>ATYAAASSALVPRGSHMYAPKLQGPVAVYTWEGNQVNITCEVFAYPSATISWFRDGQLLPSSNYSNIKI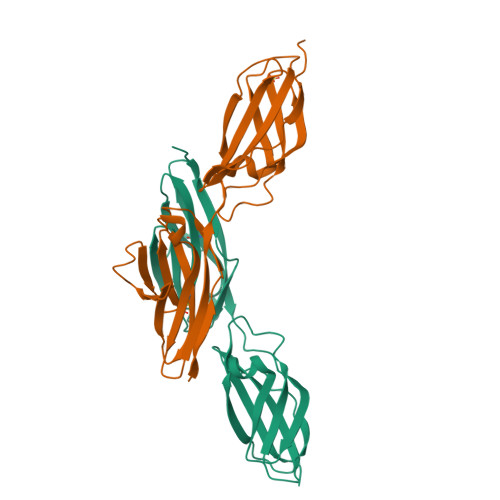YNTPSASYLEVTPDSENDFGNYNCTAVNRIGQESLEFILVQADTPSSPSIDQVEPYSSTAQVQFDEPEATGGVPILKYKAEWRAVGEEVWHSKWYDAKEASMEGIVTIVGLKPETTYAVRLAALNGKGLGEISAASEFKTQPVQGE[2x]>MARGPGLAPPPLRLPLLLLVLAAVTGHTAAQDNCTCPTNKMTVCSPDGPGGRCQCRALGSGMAVDCSTLTSKCLLLKARMSAPKNARTLVRPSEHALVDNDGLYDPDCDPEGRFKARQCNQTSVCWCVNSVGVRRTDKGDLSLRCDELVRTHHILIDLRHRPTAGAFNHSDLDAELRRLFRERYRLHPKFVAAVHYEQPTIQIELRQNTSQKAAGDVDIGDAAYYFERDIKGESLFQGRGGLDLRVRGEPLQVERTLIYYLDEIPPKFSMKRLTAGLIAVIVVVVVALVAGMAVLVITNRRKSGKYKKVEIKELGELRKEPSL[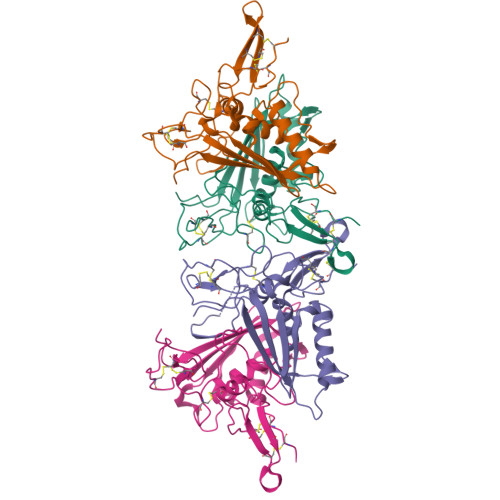4x]>LGTNYLLSGQTLNTDGHLKNGDFDLVMQNDCNLVLYNGNWQSNTANNGRDCKLTLTDYGELVIKNGDGSTVWRSRAKSVKGNYAAVLHPDGRLVVFGPSVFKIDPWVPGL[4x];>[4x]NIPFTDNLLFSGQVLYGDGRLTAKNHQLVMQG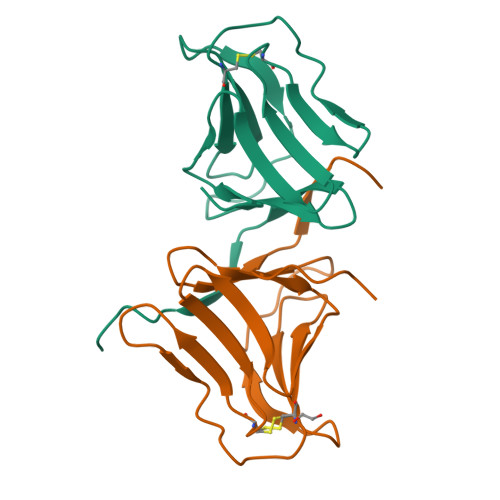DCNLVLYGGKYGWQSNTHGNGEHCFLRLNHKGELIIKDDDFKTIWSSNSSSKQGDYVLILRDDGFAVIYGPAIWETSA>[4x]MPKRTDIKSILILGAGPIVIGQACEFDYSGAQACKALREEGYRVILVNSNPATIMTDPEMADATYIEPIHWEVVRKIIEKERPDAVLPTMGGQTALNCALELERQGVLEEFGVTMIGATADAIDKAEDRRRFDVAMKKIGLETARSGIAHTMEEALAVAADVGFPCIIRPSFTMGGSGGGIAYNREEFEEICARGLDLSPTKELLIDESLIGWKEYEMEVVRDKNDNCIIVCSIENFDAMGIHTGDSITVAPAQTLTDKEYQIMRNASMAVLREIGVETGGSNVQFAVNPKNGRLIVIEMNPRVSRSSALASKATGFPIAKVAAKLAVGYTLDELMNDITGGRTPASFEPSIDYVVTKIPRFNFEKFAGANDRLTTQMKSVGEVMAIGRTQQESLQKALRGLEVGATGFDPKVSLDDPEALTKIRRELKDAGADRIWYIADAFRAGLSVDGVFNLTNIDRWFLVQIEELVRLEEKVAEVGITGLNADFLRQLKRKGFADARLAKLAGVREAEIRKLRDQYDLHPVYKRVDTCAAEFATDTAYMYSTYEEECEANPSTDREKIMVLGGGPNRIGQGIEFDYCCVHASLALREDGYETIMVNCNPETVSTDYDTSDRLYFEPVTLEDVLEIVRIEKPKGVIVQYGGQTPLKLARALEAAGVPVIGTSPDAIDRAEDRERFQHAVERLKLKQPANATVTAIEMAVEKAKEIGYPLVVRPSYVLGGRAMEIVYDEADLRRYFQTAVSVSNDAPVLLDHFLDDAVEVDVDAICDGEMVLIGGIMEHIEQAGVHSGDSACSLPAYTLSQEIQDVMRQQVQKLAFELQVRGLMNVQFAVKNNEVYLIEVNPRAARTVPFVSKATGVPLAKVAARVMAGKSLAEQGVTKEVIPPYYSVKEVVLPF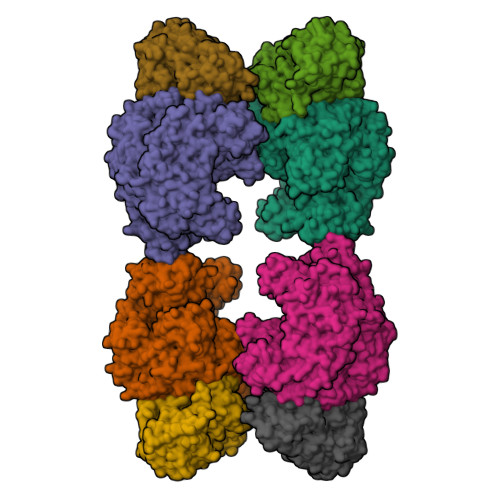NKFPGVDPLLGPEMRSTGEVMGVGRTFAEAFAKAQLGSNSTMKKHGRALLSVREGDKERVVDLAAKLLKQGFELDATHGTAIVLGEAGINPRLVNKVHEGRPHIQDRIKNGEYTYIINTTSGRRAIEDSRVIRRSALQYKVHYDTTLNGGFATAMALNADATEKVISVQEMHAQIK;>[4x]MIKSALLVLEDGTQFHGRAIGATGSAVGEVVFNTSMTGYQEILTDPSYSRQIVTLTYPHIGNVGTNDADEESSQVHAQGLVIRDLPLIASNFRNTEDLSSYLKRHNIVAIADIDTRKLTRLLREKGAQNGCIIAGDNPDAALALEKARAFPGLNGMDLAKEVTTAEAYSWTQGSWTLTGGLPEAKKEDELPFHVVAYDFGAKRNILRMLVDRGCRLTIVPAQTSAEDVLKMNPDGIFLSNGPGDPAPCDYAITAIQKFLETDIPVFGISLGHQLLALASGAKTVKMKFGHHGGNHPVKDVEKNVVMITAQNHGFAVDEATLPANLRVTHKSLFDGTLQGIHRTDKPAFSFQGHPEASPGPHDAAPLFDHFIELIEQYRKTAK> MTNTIKINSLTIAFVGALSSMGVQAHGWVEYPSARQNTCYLDGGFWDNTIPNQACQSAFDESGAFPFVQRNEVAANVPNYKDMAHVQAIVRDGNLCSAGDKAKSGLNMGSTHWQKTAITLDENNQLELVFNATAPHNPSYWQFYLSNVNYDPTVPLTWGDLDVVDTAGDIIVGDDKKYRIKITLPADRADSAVLYTRWQREDAAGEGFYNCSDIAFDGAGTTPPGPIDPVEPPPQYSDLGYYIGQGFGPVESGDSV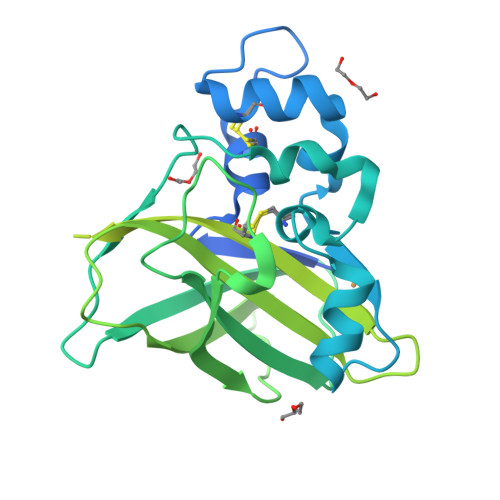RFRTFDATGAETTDISLAITVNNTATWSAELAGQFNQLKNKAWFIGIWHQEMNHYMYDTINIYANRVFAPKANLSYQLSLIKADITPPVEPPVEPTNQWDKNNAYQARESVTHQGGTWVAQWWTKGEEPGKTGEWGVWR> GPETLCGAELVDALQFVCGDRGFYFNKPTGYGSSSRRAPQTGIVDE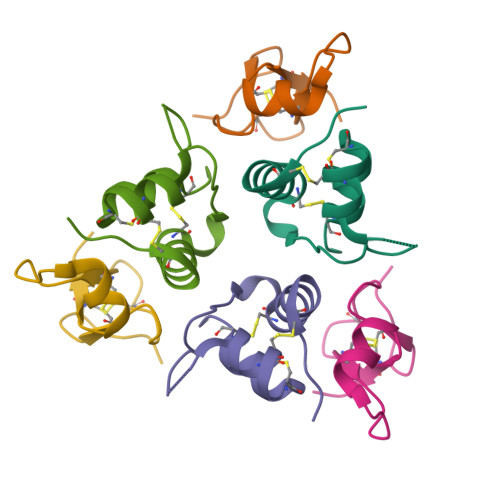CCFRSCDLRRLEMYCAPLKPAKSA;> SALAEGQSCGVYTERCAQGLRCLPRQDEEKPLHALLHGRGVCLNEKSYREQVKI>[2x]GPMATRGRPRAFDRDTALQRAMDVFWVRGYEGASLAALTEAMEIRPPSLYAAFGSKEGLFREALAHYLGQHGRYRRDVLDGAPSAREGVAELLRETVARFTSDEFPRGS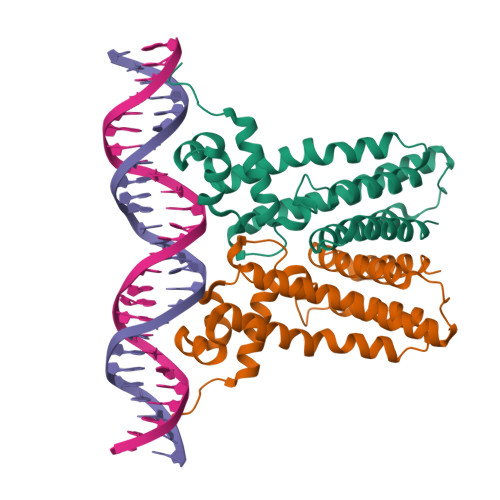LVVLAALTGTPESEAVRDALSAERGESIRLFRERMRRGIADGDLAADTDMEELATFYATVLFGLSVQAKDRVPRERLLAVVERALRAWP> MKTEW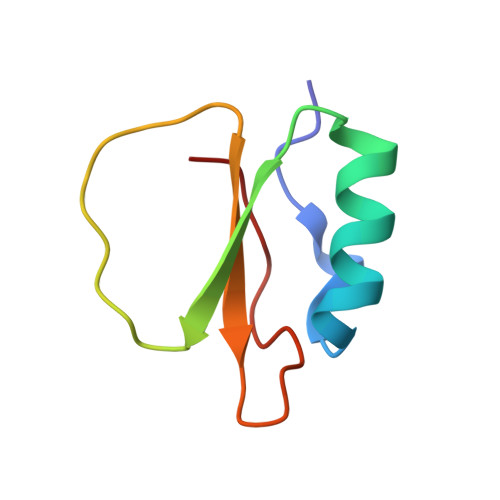PELVGKSVEEAKKVILQDKPEAQIIVLPVGTIVTMEYRIDRVRLFVDKLDNVAQVPRVG>MDFSRNLYDIGEQLDSEDLASLKFLSLDYIPQRKQEPIKDALMLFQRLQEKRMLEESNLSFLKELLFRINRLDLLITYLNTRKEEMERELQTPGRAQISAYRVMLYQISEEVSRSELRSFKGGLQEEISKCKLDDDMNLLDIFIEMEKRVILGEGKLDILKRVCAQINKSLLKIINDYEEFSKERSSSLEGSPDEFSNGEELCGVMTISDSPREQDSESQTLDKVYQMKSKPRGYCLIINNHNFAKAREKVPKLHSIRDRNGTHLDAGALTTTFEELHFEIKPHDDCTVEQIYEILKIYQLMDHSNMDCFICCILSHGDKGIIYGTDGQEAPIYELTSQFTGLKCPSLAGKPKVFFIQAAQGDNYQKGIPVETASEEQPYLEMALSSPQTRYIPDEADFLLGMATVNNCVSYRNPAEGTWYIQSLCQSLRERCPRGDDILTILTEVNYEVSNKDDKKNMGKQMPQPTFTLRKKLVFPSD[3x];>MSAEVIHQVEEALDTDEKEMLLFLCRDVAIDVVPPNVRDLLDILRERGKLSVGDLAELLYRVRRFDLLKRILKMDRKAVETHLLRNPHLVSDYRVLMAEIGEDLDKSDVSSLIFL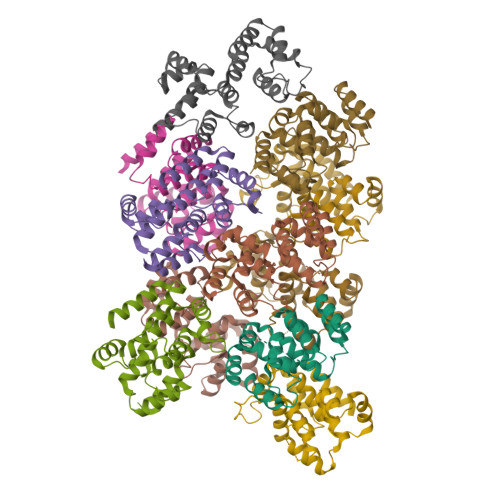MKDYMGRGKISKEKSFLDLVVELEKLNLVAPDQLDLLEKCLKNIHRIDLKTKIQKYKQSVQGAGTS[8x]>VSEDLRSRIEVLKRKVIEKVQHIQLLQKNVRAQLVDMKRLEVDIDIKIRSCRGSCSRALAREVDLKDYEDQQKQLEQVIAKDLLPSR[2x];>DNENVVNEYSSELEKHQLYIDETVNSNIPTNLRVLRSILENLRSKIQKLESDVSAQMEYCRTPCTVSCNIPVVSGKECEEIIRKGGETSEMYLIQPDSSVKPYRVYCDMNTENGGWTVIQNRQDGSVDFGRKWDPYKQGFGNVATNTDGKNYCGLPGEYWLGNDKISQLTRMGPTELLIEMEDWKGDKVKAHYGGFTVQNEANKYQISVNKYRGTAGNALMDGASQLMGENRTMTIHNGMFFSTYDRDNDGWLTSDPRKQCSKEDGGGWWYNRCHAANPNGRYYWGGQYTWDMAKHGTADGVVWMNWKGSWYSMRKMSMKIRPFFPQQ[2x];>[2x]KMLEEIMKYEASILTHDSSIRYLQEIYNSNNQKIVNLKEKVAQLEAQCQEPCKDTVQIHDITGKDCQDIANKGAKQSGLYFIKPLKANQQFLVYCEIDGSGNGWTVFQKRLDGSVDFKKNWIQYKEGFGHLSPTGTTEFWLGNEKIHLISTQSAIPYALRVELEDWNGRTSTADYAMFKVGPEADKYRLTYAYFAGGDAGDAFDGFDFGDDPSDKFFTSHNGMQFSTWDNDNDKFEGNCAEQDGSGWWMNKCHAGHLNGVYYQGGTYSKASTPNGYDNGIIWATWKTRWYSMKKTTMKIIPFN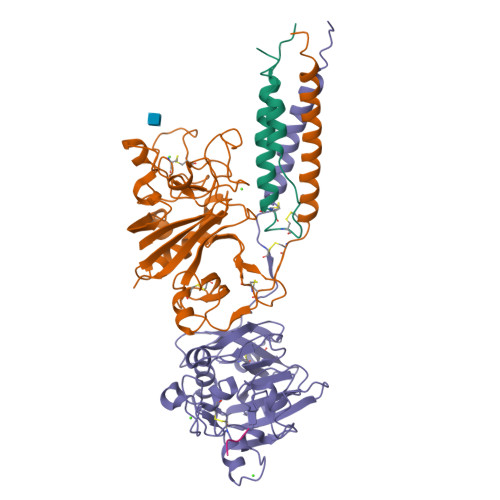RLTIGEGQQHHLGGAK;>GHRPX[2x]>MSEGEGQAKNRLFLGVDLGTSHTAVMSSRGKKFLLKSVVGYPKDVIGLKLLGRPYVVGDEAFEMRSYLDIRYPLQDGVLSEISDRDIEVARHLLTHVVKSAEPGPNDEICAVIGVPARASAANKALLLKMAQEVVHTALVVSEPFMVGYGLDKLINTIIVDIGAGTTDICALKGTVPGPEDQVTLTKAGNYVDERLQNAILERHPELQMNVNVACAVKEQFSFVGTPTEVASFEFRAAGKPVRADVTEPVKIACEALMPDIIESIETLLRSFQPEYQATVLQNIVFAGGGSRIRGLAAYVKEKLRPFGDANVTCVKDP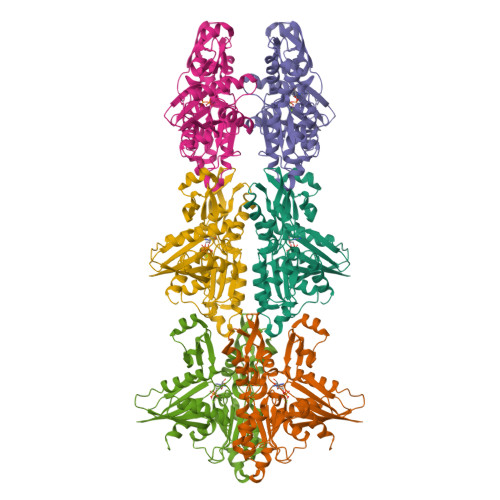TFDGCRGALRLAEELPPQYWRQLGDVSGS[6x]>[5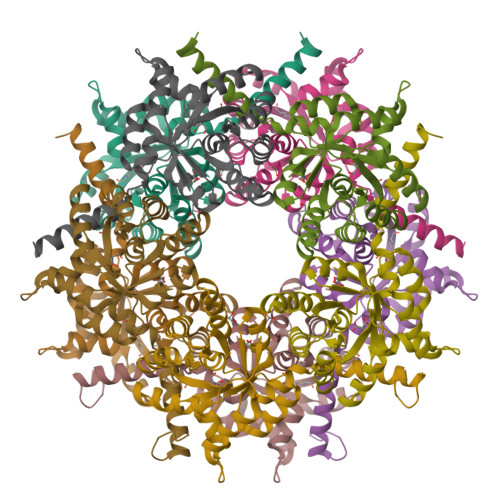x]MKIFLDTANIDEIRTGVNWGIVDGVTTNPTLISKEAVNGKKYGDIIREILKIVDGPVSVEVVSTKYEGMVEEARKIHGLGDNAVVKIPMTEDGLRAIKTLSSEHINTNCTLVFNPIQALLAAKAGVTYVSPFVGRLDDIGEDGMQIIDMIRTIFNNYIIKTQILVASIRNPIHVLRSAVIGADVVTVPFNVLKSLMKHPKTDEGLAKFLEAWKKVSPDGKLIL> MKVLVPVKRLIDYNVKARVKSDGSGVDLANVKMSMNPFDE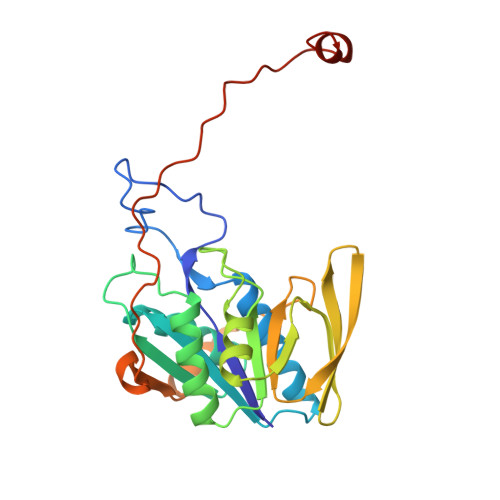IAVEEAIRLKEKGQAEEIIAVSIGVKQAAETLRTALAMGADRAILVVAADDVQQDIEPLAVAKILAAVARAEGTELIIAGKQAIDNDMNATGQMLAAILGWAQATFASKVEIEGAKAKVTREVDGGLQTIAVSLPAVVTADLRLNEPRYASLPNIMKAKKKPLDEKTAADYGVDVAPRLEVVSVREPEGRKAGIKVGSVDELVGKLKEAGVI> TLHDKQIRICHLFEQLSSATVIGDGDKHKHSDRLKNVGKLQPGAIFSCFHPDHLEEARHLYEVFWEAGDFNDFIEIAKEARTFVNEGLFAFAAEVAVLHRDDCKGLYVPPVQEIFPDKFIPSAAINEAFKKAHVRPEFDESPILVDVQDTGNILDPEYRLAYYREDVGINAHHWHWHLVYPSTWNPKYFGKKKDRKGELFYYMHQQMCARYDCERLSNGMHRMLPFNNFDEPLAGYAPHLTHVASGKYYSPRPDGLKLRDLGDIEISEMVRMRERILDSIHLGYVISEDGSHKTLDELHGTDILGALVESSYESVNHEYYGNLHNWGHVTMARIHDPDGRFHEEPGVMSDTSTSLRDPIFYNWHRFIDNIFHEYKNTLKPYDHDVLNFPDIQVQDVTLHARVDNVVHTFMREQELELKHGINPGNARSIKAKYYHLDHEPFSYAVNVQNNSASDKHATVRIFLAPKYDELGNEIKADELRRTAIELDKFKTDLHPGKNTVVRHSLDSSVTLSHQ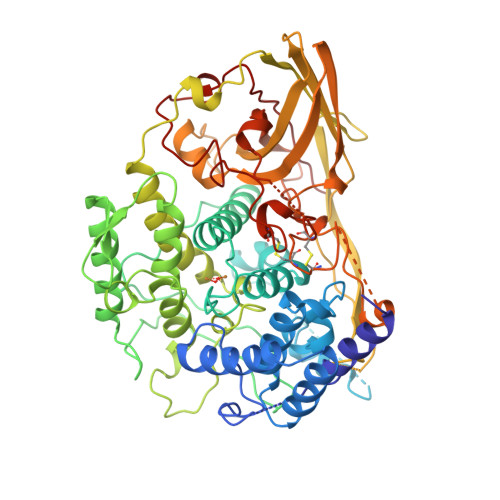PTFEDLLHGVGLNEHKSEYCSCGWPSHLLVPKGNVAGMEYHLFVMLTDWDKDKVDGSESVACVDAVSYCGARDHKYPDKKPMGFPFDRPIHTEHISDFLTNNMFIKDIKIKFHE>[2x]GTVWGALGHGINLNIPNFQMTDDIDEVRWERGSTLVAEFKRKPFLKSGAFEIL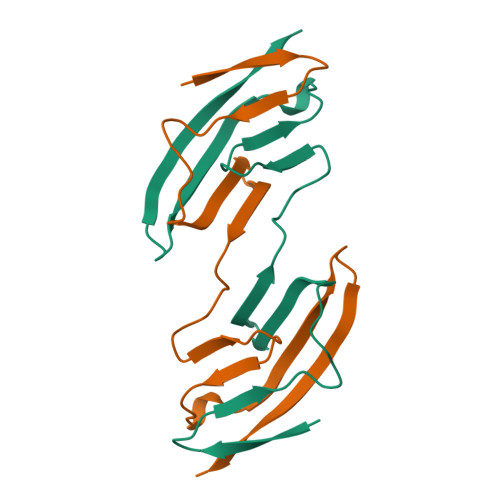ANGDLKIKNLTRDDSGTYNVTVYSTNGTRILDKALDLRILE> MSIQAFVFCGKGSNLAPFTQPDFPFQTQNKDSTAATSGDKLNELVNSALDSTVINEFMQHSTRLPKALLPIGNRPMIEYVLDWCDQADFKEISVVAPVDEIELIESGLTSFLSLRKQQFELIYKALSNSNHSHHLQDPKKINFIPSKANSTGESLQKELLPRINGDFVILPCDFVTDIPPQVLVDQFRNRDDNNLAMTIYYKNSLDSSIDKKQQQKQKQQQFFTVYSENEDSERQPILLDVYSQRDVTKTKYLQIRSHLLWNYPNLTVSTKLLNSFIYFCSFELCQLLKLGPQSMSRQASFKDPFTGNQQQQNPPTTDDDEDRNHDDDDDYKPSATSIQPTYFKKKNDLILDPINCNKSLSKVFRDLSRRSWQHSKPREPIGIFILPNETLFIRANNLNAYMDANRFVLKIKSQTMFTKNIQIQSAAIGADAIVDPKCQISAHSNVKMSVLGTQANIGSRCRVAGSLLFPGVHLGDEVILENCI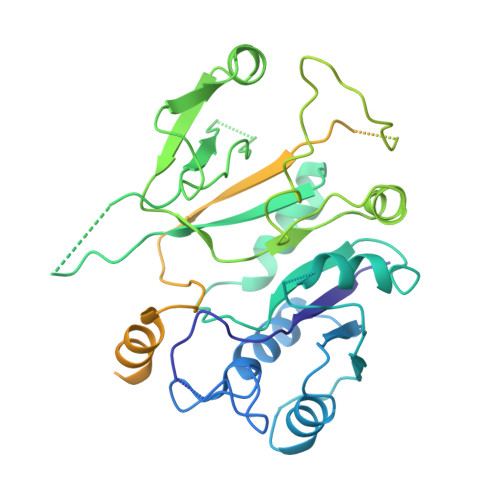IGPMAKIGSKCKLSNCYIEGHYVVEPKNNFKGETLANVYLDEDEEDELIYDDSVIAGESEIAEETDSDDRSDEDSDDSEYTDEYEYEDDGLFER2-methylpropyl 5-[(3aS,4S,6aR)-2-oxohexahydro-1H-thieno[3,4-d]imidazol-4-yl]pentanoate | C14 H24 N2 O3 S | 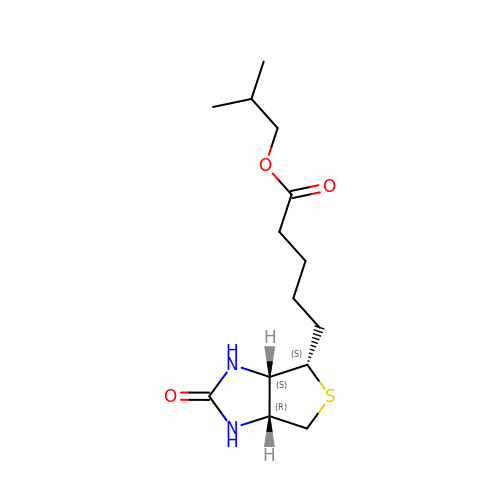TYWDFVAUHFABAM-GVXVVHGQSA-N> MPQSSSADRLSRPFTEAAATRLNRWPAFPYHVWVRVSLWVSVVTVAALFGWGAWQRRWIADDGLIVLRTVRNLLAGNGPVFNAGERVEANTSTVWSYLVTLGGFVAGSARLEYVALVLALTLSVLGVVLVMFGTARLYAPGLTGRRAVFLPAGALVYIAIPPARDFATSGLENGLVLAYLGLLWWMMVCWSQGLRRPDGERTSRGFDATLAVVAGMSVLVRPELALIGGLALVMMLVAAPTWRRRLALVVVGGLIPVAYQIFRMGYYGLLVPGTALAKDASGAKWDQGLVYLANFNQPYLLW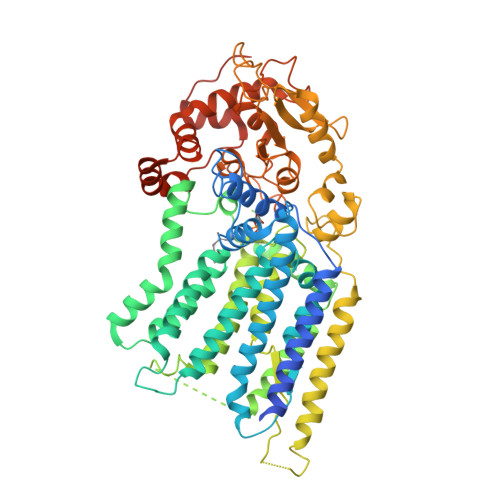APAVLLIGLGLMVLLLRGRPSWGDRGARKESGWIARTVQSPPAVVAFMLISGLLQAVYWIRQGGDFMHGRVLLTPLFCLLAPVAVIPLLLPDRSRMARGAGYLYAGATAVLWLAVAGWALWAANSPGMGADATRVTYSGIVDERRFYSQATGHAHPLTAADYLDYPRMRAVLTAIENTPDGALLLPSGDYDRWDVVPALPPPPDVRAAAVGGYVGPHTVFFTNLGMLGMNVGLDVRVIDQIGLANPLAAHTARLTDGRIGHDKNLFPDWAVAEGPFLKEPPWIPQYLDEDWIRQAEAALKCPETDKVLDAIRAPMGFRRFLSNVMHAAEYTRYRIDRVPLYELARCGLPVPEPVDPPYTGLPPTGPA>MESLPVIAAPSMWTRPQIKDFKEKIRQDADSVITVGRGEVVTVRVPTHEEGSYLFWEFATDNYDIGFGVYFEWTDSPNTAVSVHVSESSDDDEEEEENISSEEKAKKNANKPLLDEIVPVYRRDCHEEVYAGSHQYP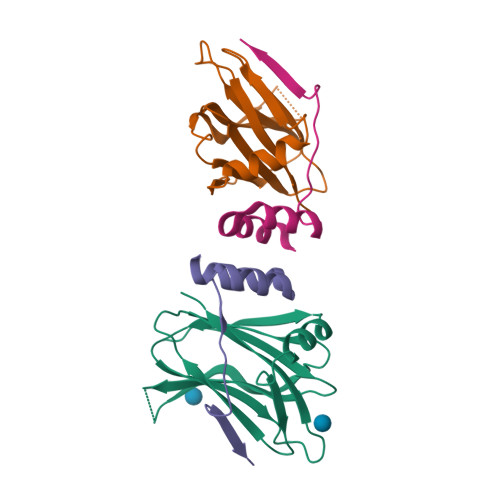GRGVYLLKFDNSYSLWRSKSVYYRVYYTR[2x];>GSGSGTPAPPAIADLLASVDSEEVRDYCRTKGWIVQEKITKESLERNVNR[2x]> GPVEDAITAAIGRVADTVGTGPTNSEAIPALTAAETGHTSQVVPGDTMQTRHVKNYHSRSESTIENFLCRSACVYFTEYENSGAKRYAEW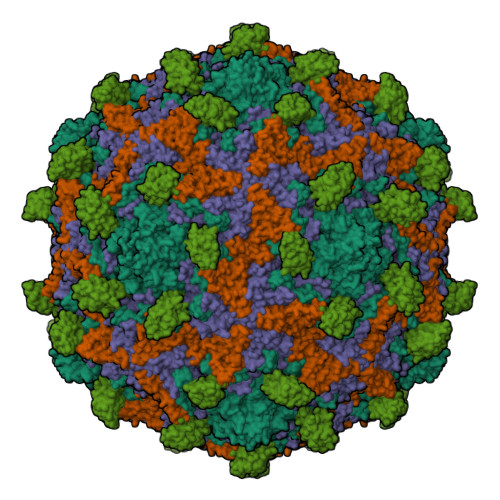VLTPRQAAQLRRKLEFFTYVRFDLELTFVITSTQQPSTTQNQDAQILTHQIMYVPPGGPVPDKVDSYVWQTSTNPSVFWTEGNAPPRMSIPFLSIGNAYSNFYDGWSEFSRNGVYGINTLNNMGTLYARHVNAGSTGPIKSTIRIYFKPKHVKAWIPRPPRLCQYEKAKNVNFQPSGVTTTRQSITTMTNT;> SPTVEECGYSDRARSITLGNSTITTQECANVVVGYGVWPDYLKDSEATAEDQPTQPDVATCRFYTLDSVQWQKTSPGWWWKLPDALSNLGLFGQNMQYHYLGRTGYTVHVQCNASKFHQGCLLVVCVPEAEMGCATLDNTPSSAELLGGDSAKEFADKPVASGSNKLVQRVVYNAGMGVGVGNLTIFPHQWINLRTNNSATIVMPYTNSVPMDNMFRHNNVTLMVIPFVPLDYCPGSTTYVPITVTIAPMCAEYNGLRLAGHQ;> GLPTMNTPGSCQFLTSDDFQSPSAMPQYDVTPEMRIPGEVKNLMEIAEVDSVVPVQNVGEKVNSMEAYQIPVRSNEGSGTQVFGFPLQPGYSSVFSRTLLGEILNYYTHWSGSIKLTFMFCGSAMATGKFLLAYSPPGAGAPTKRVDAMLGTHVVWDVGLQSSCVLCIPWISQTHYRYVTSDEYTAGGFITCWYQTNIVVPADAQSSCYIMCFVSACNDFSVRLLKDTPFISQQNFFQ;> MGAQVSTQKTGAHETGLNASGNSIIHYTNINYYKDAASNSANRQDFTQDPGKFTEPVKDIMIKSLPALN;> MSITTPEEMIEKAKGETAYLPCKFTLSPEDQGPLDIEWLISPADNQKVDQVIILYSGDKIYDDYYPDLKGRVHFTSNDLKSGDASINVTNLQLSDIGTYQCKVKKAPGVANKKIHLVVLVKPSGARCYVDGSEEIGSDFKIKCEPKEGSLPLQYEWQKLSDSQKMPTSWLAEMTSSVISVKNASSEYSGTYSCTVRNRVGSDQCLLRLNVVPPSNKALEHHHHHH COPROPORPHYRINOGEN III | C36 H44 N4 O8 | 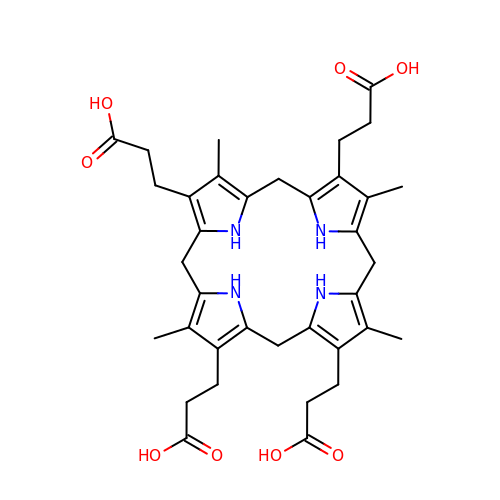NIUVHXTXUXOFEB-UHFFFAOYSA-N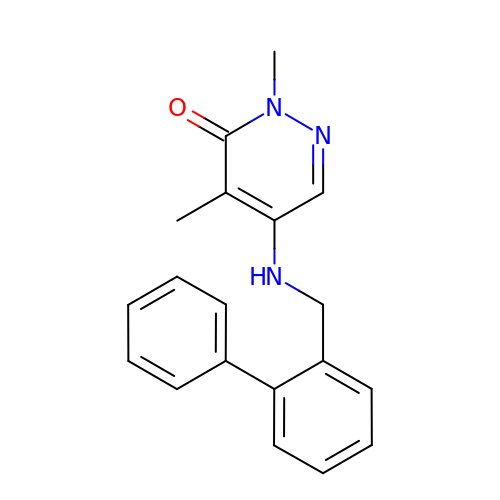2,4-dimethyl-5-[(2-phenylphenyl)methylamino]pyridazin-3-one | C19 H19 N3 O | JLOICACPNWZYGI-UHFFFAOYSA-N>[8x]AKHQERVQRLKEECEAGSRELKRCK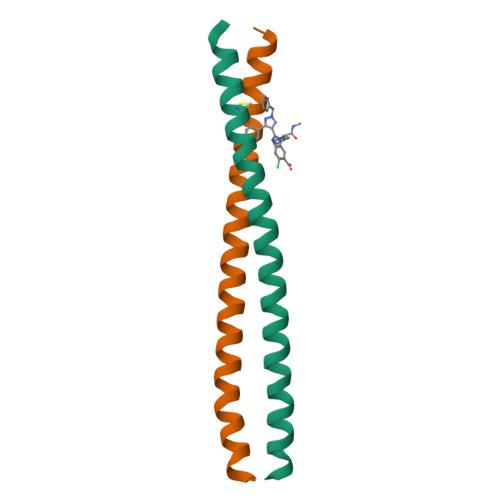EENYDLAMRLAHQSEEKGAALMRNRDLQLEIDQLK> MKKIILTIGCPGSGKSTWAREFIAKNPGFYNINRDDYRQSIMAHEERDEYKYTKKKEGIVTGMQFDTAKSILYGGDSVKGVIISDTNL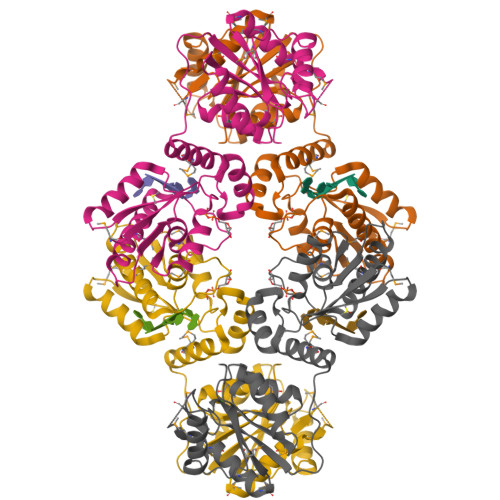NPERRLAWETFAKEYGWKVEHKVFDVPWTELVKRNSKRGTKAVPIDVLRSMYKSMREYLGLPVYNGTPGKPKAVIFDVDGTLAKMNGRGPYDLEKCDTDVINPMVVELSKMYALMGYQIVVVSGRESGTKEDPTKYYRMTRKWVEDIAGVPLVMQCQREQGDTRKDDVVKEEIFWKHIAPHFDVKLAIDDRTQVVEMWRRIGVECWQVASGDF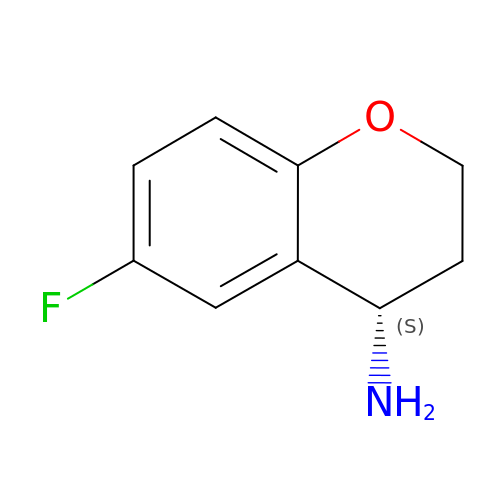(4~{S})-6-fluoranyl-3,4-dihydro-2~{H}-chromen-4-amine | C9 H10 F N O | WVQYSVLMDHXHOV-QMMMGPOBSA-N>[24x]GPMSDEQTFIAIKPDGVQRGLVGPIISRFENRGFKLAALKLCSPSKEHLEQHYADLSSKPFFPGLVSYMLSGPIVAMVWEGREVVKTGRTILGATN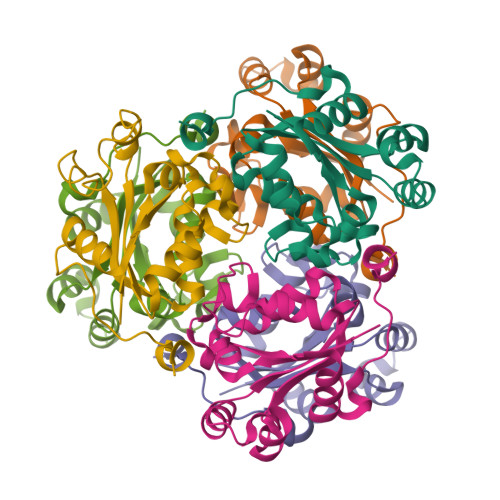PLASAPGTIRGDFAIDVGRNVCHGSDSVENAKKEIALWFKPEELQKYKHSQFDWIYEKA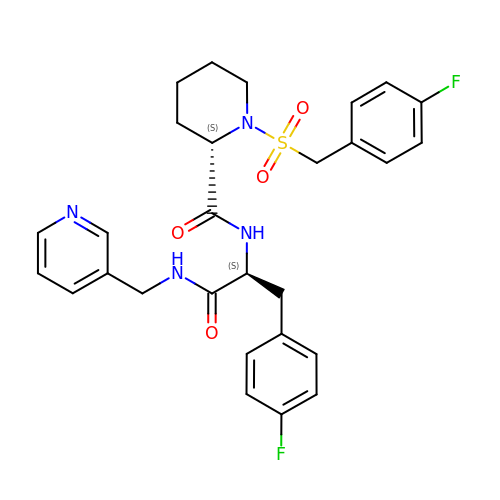(2~{S})-1-[(4-fluorophenyl)methylsulfonyl]-~{N}-[(2~{S})-3-(4-fluorophenyl)-1-oxidanylidene-1-(pyridin-3-ylmethylamino)propan-2-yl]piperidine-2-carboxamide | C28 H30 F2 N4 O4 S | FCUDWGSHVIZNIL-UIOOFZCWSA-N>GTSTQTKAGSLTIVGTGIESIGQMTLQALSYIEAAAKVFYCVIDPATEAFILTKNKNCVDLYQYYDNGKSRLNTYTQMSELMVREVRKGLDVVGVFYGHPGVFVNPSHRALAIAKSEGYRARMLPGVSAEDCLFADLCIDPSNPGCLTYEASDFLIRDRPVSIHSHLVLFQVGCVGIADFNFTGFDNNKFGVLVDRLEQEYGAEHPVVHYIAAMMPHQDPVTDKYTVAQLREPEIAKRVGGVSTFYIPPKARKASNLDIIRRLELLPAGQVPDKKARIYPANQWEPDVPEVEPYRPSDQAAIAQLADHAPPEQYQPLATSKAMSDVMTKLALDPKALADYKADHRAFAQSVPDLTPQERAALELGDSWAIRCAMKNMPSSLLDAARES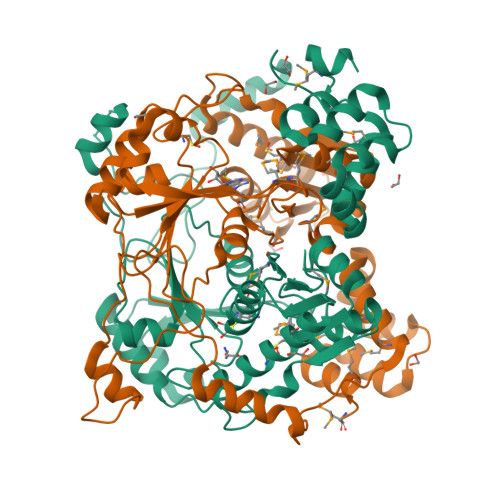GEEASQNGFP[2x]>[2x]MGGSHHHHHHGTMKQLISLKNIFRSYRNGDQELQVLKNINLEVNEGEFVAIMGPSGSGKSTLMNTIGMLDTPTSGEYYLEGQEVAGLGEKQLAKVRNQQIGFVFQQFFLLSKLNALQNVELPLIYAGVSSSKRRKLAEEYLDKVELTERSHHLPSELSGGQKQRVAIARALVNNPSIILADEPTGALDTKTGNQIMQLLVDLNKEGKTIIMVTHEPEIAAYAKRQIVIRDGVISSDSAQLGKEEN;>[2x]MQNLKFAFSSIMAHKMRSLLTMIGIIIGVSSVVVIMALGDSLSRQVNKDMTKSQKNISVFFSPKKSKDGSFTQKQSAFTVSGKEEEVPVEPPKPQESWVQEAAKLKGVDSYYVTNSTNAILTYQDKKVENANLTGGNRTYMDAVKNEIIAGRSLREQDFKEFASVILLDEELSISLFESPQEAINKVVEVNGFSYRVIGVYTSPEAKRSKIYGFGGLPITTNISLAANFNIDEIASIVFRVNDTSLTPTLGPELARKMTELAGLQQGEYQVADESVVFAEIQQSFSFMTTIISSIAGISLFVGGTGVMNIMLVSVTERTREIGLRKALGATRANILIQFLIESMILTLLGGLIGLTIASGLTALAGLLLQGLIEGIEVGVSIPVALFSLAVSASVGMIFGVLPANKASKLDPIEALRYE

The operon spr0693-spr0694-spr0695 of S. pneumoniae R6 encodes a putative ABC transporter that contributes to the resistance of antibiotics and antimicrobial peptides. Sequence analyses suggest that the Spr0693–0694–0695 assembly is similar to Escherichia coli MacAB, with Spr0693 and Spr0694–0695 corresponding to MacA and MacB, respectively. Here we present the crystal structures of S. pneumoniae Spr0694–0695 and Spr0693, representing the structure of a MacAB-like efflux pump in Gram-positive bacteria. In summary, the structure of Spr0694-Spr0695 reveals some features for this family of ABC transporters, which are characterized by a unique 8-TM fold and an ECD/PLD insertion between TM1 and TM2.

The crystal structure of Spr0694–0695 was determined at 3.3 Å resolution. Each asymmetric unit contains an ABC transporter with a pseudo two-fold symmetry, the NBD and TMD of which are encoded by spr0694 and spr0695, respectively. Spr0695/TMD could be further divided into two domains, a 4-TM helical bundle and an extracellular domain (ECD) inserted between TM1 and TM2. Notably, each TMD subunit has only four transmembrane (TM) helices, which is distinct from the TMD of canonical exporters that usually possesses six TM helices. The two discrete 4-TM bundles are folded in a back-to-back manner, without domain swapping usually applied in other ABC transporters, especially in type I exporters. In contrast, the TMDs buried in the membrane pack against each other tightly via hydrophobic interactions with a buried interface of ~1800 Å2, leaving no opening to the intracellular face of the membrane. Notably, a short helix α6 (residues Pro204–Tyr212) of the ESM, which is located at the interface between the ECD and TMD, sticks to the TM helices via hydrophobic interactions and four salt bridges: Lys207 and Lys210–Glu374, Arg208-Asp49 and Glu205–Lys52. The two NBD subunits are somewhat separated, leaving the ATP-binding pocket exposed to the solvent. However, the nucleotide is absent from the electron density map, despite the protein was co-crystallized with ATP analog AMP-PNP. Thus, we propose that the helix α6 functions as a guard at the entrance of substrate tunnel, thus terming it the guard helix.> MSETSFNLISEKC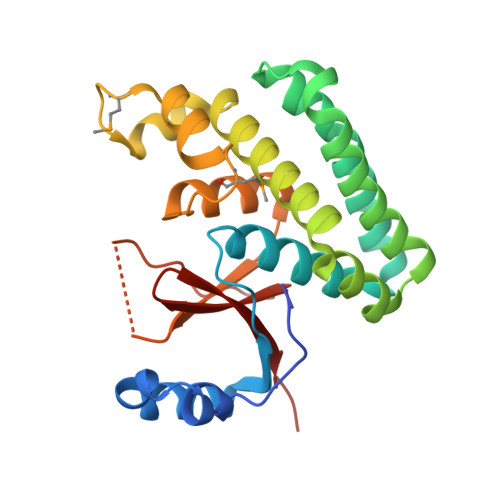DILSILRDHPENRIYRRKIEELSKRFTAIRKTKGDRNCFYRALGYSYLESLLGKSREIFKFKERVLQTPNDLLAAGFEEHKFRNFFNAFYSVVELVEKDGSVSSLLKVFNDQSASDHIVQFLRLLTSAFIRNRADFFRHFIDEEMDIKDFCTHEVEPMATECDHIQITALSQALSIALQVEYVDEMDTALNHHVFPEAATPSVYLLYKTSHYNILYAADKH>[60x]MNNLYRDLAPVTEAAWAEIELEAARTFKRHIAGRRVVDVSDPGGPVTAAVSTGRLIDVKAPTNGVIAHLRASKPLVRLRVPFTLSRNEIDDVERGSKDSDWEPVKEAAKKLAFVEDRTIFEGYSAASIEGIRSASSNPALTLPEDPREIPDVISQALSELRLAGVDGPYSVLLSADVYTKVSETSDHGYPIREHLNRLVDGDIIWAPAIDGA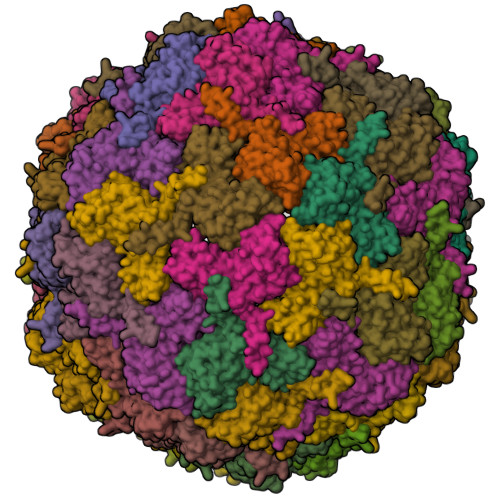FVLTTRGGDFDLQLGTDVAIGYASHDTDTVRLYLQETLTFLCYTAEASVALSH>MLNPQLVQPAKKPYNKIVSHLLVAEPEKIYAMPDPTVPDSDIKALTTLCDLADRELVVIIGWAKHIPGFSTLSLADQMSLLQSAWMEILILGVVYRSLSFEDELVYADDYIMDEDQSKLAGLLDLNNAILQLVKKYKSMKLEKEEFVTLKAIALANSDSMHIEDVEAVQKLQDVLHEALQDYEAGQHMEDPRRAGKMLMTLPLLRQTSTKAVQHFYNIK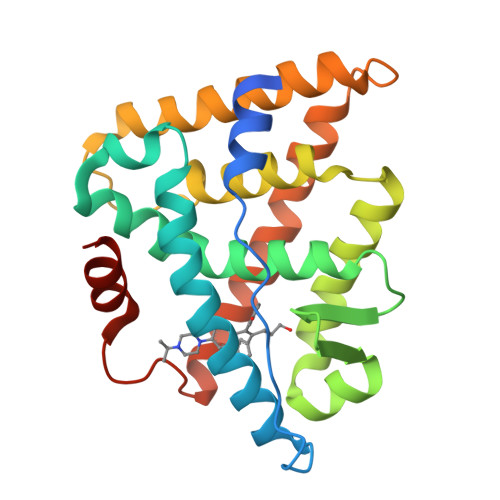LEGKVPMHKLFLEMLEAKV[3x]>MRLPVSFPLTVLSLLGSTIAHPYGETEAVLRSEPKSNQAKADAVKEAFQHAWNGYMKYAFPHDELTPVSNGHADSRNGWGASAVDALSTAVIMGKADVVNAILEHVADIDFSKTSDTVSLFETTIRYLAGMLSGYDLLQGPAKNLVDNQDLIDGLLDQSRNLADVLKFAFDTPSGVPYNNINITSHGNDGATTNGLAVTGTLVLEWTRLSDLTGDEEYAKLSQKAESYLLKPQPSSSEPFPGLVGSSININDGQFADSRVSWNGGDDSFYEYLIKMYVYDPKRFETYKDRWVLAAESTIKHLKSHPKSRPDLTFLSSYSNRNYDLSSQHLTCFDGGSFLLGGTVLDRQDFIDFGLELVDGCEATYNSTLTKIGPDSWGWDPKKVPSDQKEFYEKAGFYISSGSYVLRPEVIESFYYAHRVTGKEIYRDWVWNAFVA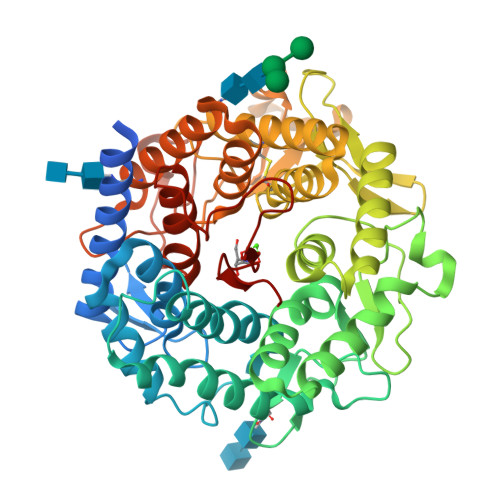INSTCRTDSGFAAVSDVNKANGGSKYDNQESFLFAEVMKYSYLAHSEDAAWQVQKGGKNTFVYNTEAHPISVARN[2x]>GSHMSNNALDRLINKQKPKVPPRNDVVSESVSNDIKTQGQQELNT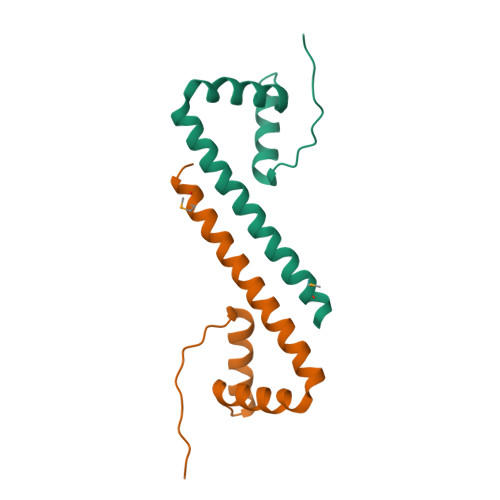SLPPSDTKATPEEMPTSHESETSLSQDQKPKLSPDTFETVRNTIRIESEVDESLRQLCHEERITKETWLEAAYLYLCEKPEELAQVIQLAQERLSQRKAIADYKRAKTMQERFL[4x]> MAHHHHHHMNASTRRPPFAGKTFEVRYDGLTALNAYDEDGRHMRYAITDGPYAGATGEVEYTWQPVAADTYAIAWQEADRATVVHIDDFAAGTSRTF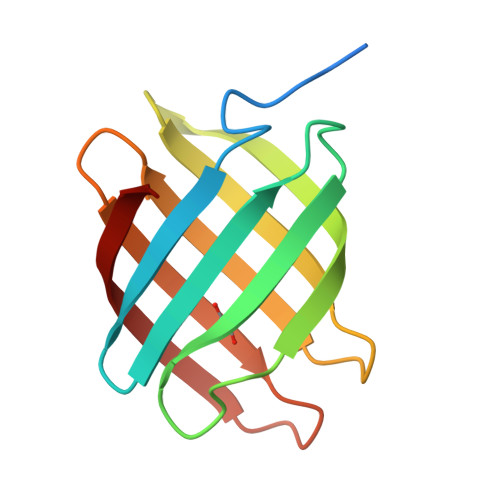FTAASLDFHRLDGSLRAV> MGEIYTETLQQTYAWTAGTNIPIKIPRNNFIRKIRVQLIGSISNSGTAAVTLPSAPFPYNL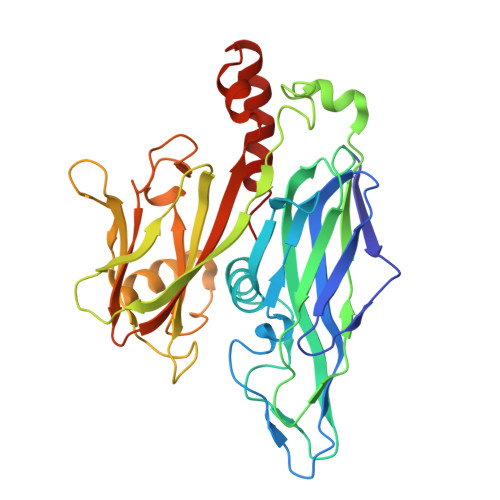VQTFNLSYEGSKTLYSVSGTGLGILMYYTTKGQNPAYPAPGTSVPASGSVNLNVMWEFDLARFPATMVQNIILSILTGQAPSGVSINASFYITITYERVTAQEILSEGGLGADGEMPLATVLPKVIEIPTFNVPASSAPIHVAYLQPGQIYKRQLVYVINSTSGINNTDPTEYELKIVRGVPTDKIKVSWAALQAENQAEYQVAPYSGASAIIDFRKYFNGDLDLTHAPSDSIEYDLALQNQDNVYSLYVSYVLPYYDQLAALPAQVAAIVQQYVARQKRRIKR Nowadays, the E3 ligase substrate receptor cereblon (CRBN), thalidomide’s primary target, is of particular importance in the fields of MGs and PROTACs. However, these CRBN ligands induce the degradation of IMiD neosubstrates and are inherently unstable, degrading hydrolytically under moderate conditions. In this work, we simultaneously optimized physiochemical properties, stability, on-target affinity, and off-target neosubstrate modulation features to develop novel nonphthalimide CRBN binders. These efforts led to the discovery of conformationally locked benzamide-type derivatives that replicate the interactions of the natural CRBN degron, exhibit enhanced chemical stability, and display a favorable selectivity profile in terms of neosubstrate recruitment.

Halo derivatives 8d (R = F) and 11a (R = Cl) could benefit from both mechanisms, haloalkyl compound 11b (R = CF3) displays strong deactivating properties, whereas compounds 11c (R = CH3), 11d (R = OMe), and 11e (R = OH) have ascending electron donating features. The inherent conformational flexibility of benzamides 11 along the amide bond was investigated using a force field-based method implemented in Schrödinger MacroModel. As expected, IMHBs were observed in low-energy conformers, except for 11a–11c. Fortunately, we could study all compounds generated in this iterative step through cocrystal structures in complex with the hTBD homolog MsCI4.44 These data confirmed that the preferred orientation of the ortho substituent toward the amide NH was preserved in the bound state of all ligands except for 11b. Sub van der Waals distances ranging from 1.3 to 2.0 Å were seen in 8d, 11a, 11c, 11d, 11e, and 11f.

>[3x]ASIFRCRQCGQTISRRDWLLPMGGDHEHVVFNPAGMIFRVWCFSLAQGLRLIGAPSGEFSWFKGYDWTIALCGQCGSHLGWHYEGGSQPQTFFGLIKDRLAEGPA> MATKLQDGNTPCLAATPSEPRPTVLVFDSGVGGLSVYDEIRHLLPDLHYIYAFDNVAFPYGEKSEAFIVERVVAIVTAVQERYPLALAVVACNTASTVSLPALREKFDFPVVGVVPAIKPAARLTANGIVGLLATRGTVKRSYTHELIARFANECQIEMLGSAEMVELAEAKLHGEDVSLDALKRILRPWLRMKEPPDTVVLGCTHFPLLQEELLQVLPEGTR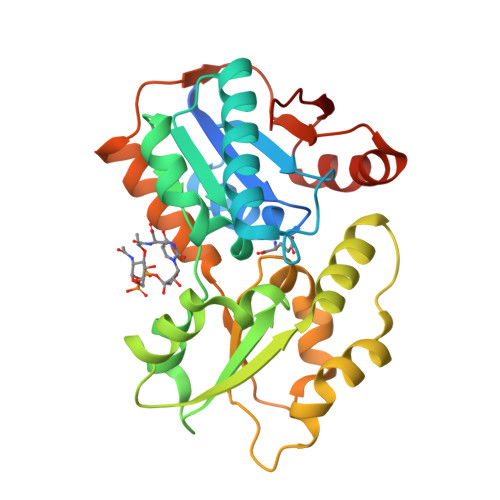LVDSGAAIARRTAWLLEHEAPDAKSADANIAFCMAMTPGAEQLLPVLQRYGFETLEKLAVLG> GSHMSGIALSRLAQERKAWRKDHPFGFVAVPTKNPDGTMNLMNWECAIPGKKGTPWEGGLFKLR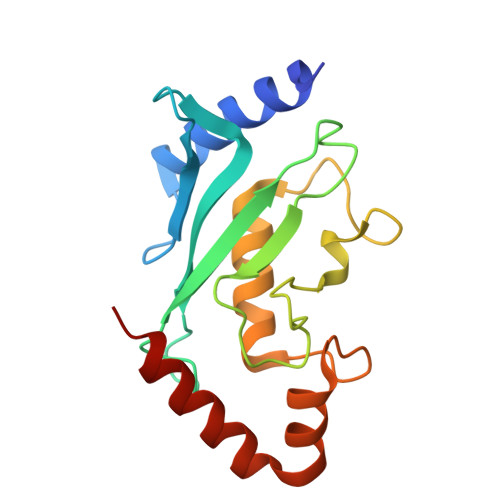MLFKDDYPSSPPKCKFEPPLFHPNVYPSGTVCLSILEEDKDWRPAITIKQILLGIQELLNEPNIQAPAQAEAYTIYCQNRVEYEKRVRAQAKKFAPS> GSVVIVGRIILSGKGGPITAYSQQTRGLLGCIITSLTGRDRNQVEGE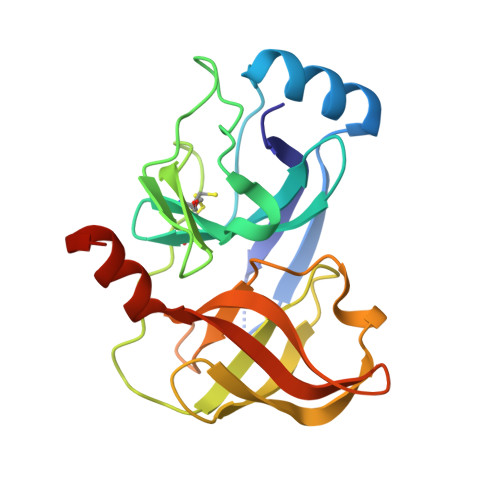VQVVSTATQSFLATCVNGVCWTVYHGAGSKTLAGPKGPITQMYTNVDQDLVGWQAPPGARSLTPCTCGSSDLYLVTRHADVIPVRRRGDSRGSLLSPRPVSYLKGSSGGPLLCPSGHAVGIFRAAVCTRGVAKAVDFVPVESMETTMRGSHHHHHH N-[1-(AMINOMETHYL)CYCLOPROPYL]-3-(MORPHOLIN-4-YLSULFONYL)-N~2~-[(1S)-2,2,2-TRIFLUORO-1-(4-FLUOROPHENYL)ETHYL]-L-ALANINAMIDE | C19 H26 F4 N4 O4 S | 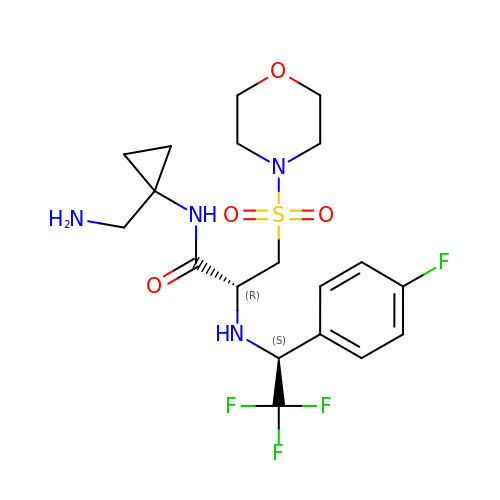BJIKKEHGGYGGIX-HOTGVXAUSA-N>GGGAAGAUAUAAUCCUAAUGAUAUGGUUUGGGAGUUUCUACCAAGAGCCUUAAACUCUUGAUUAUCUUCC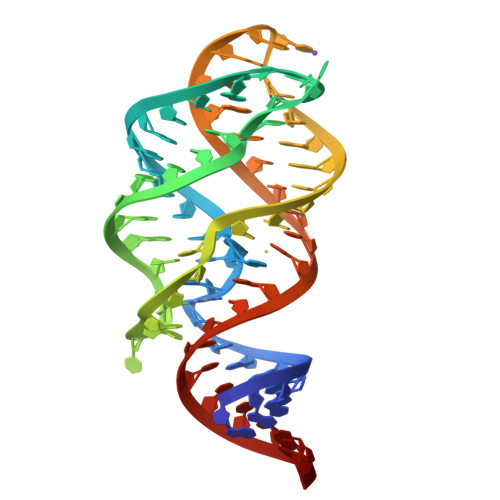C[2x]>MAVNELLHLAPNVWPRNTTRDEVGVVCIAGIPLTQLAQEYGTPLFVIDEDDFRSRCRETAAAFGSGANVHYAAKAFLCSEVARWISEEGLCLDVCTGGELAVALHASFPPERITLHGNNKSVSELTAAVKAGVGHIVVDSMTEIERLDAIAGEAGIVQDVLVRLTVGVEAHTHEFISTAHEDQKFGLSVASGAAMAAVRRVFATDHLRLVGLHSHIGSQIFDVDGFELAAHRVIGLLRDVVGEFGPEKTAQIATVDLGGGLGISYLPSDDPPPIAELAAKLGTIVSDESTAVGLPTPKLVVEPGRAIAGPGTITLYEVGTVKD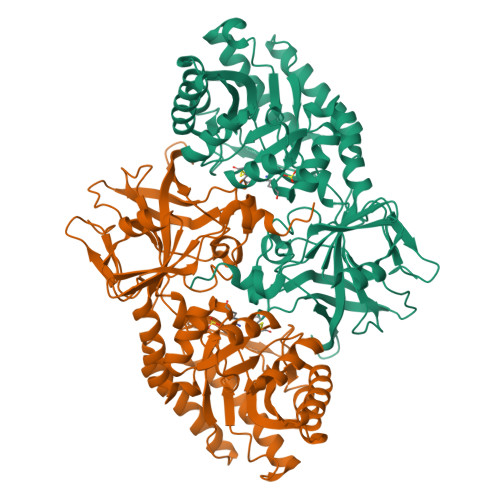VDVSATAHRRYVSVDGGMSDNIRTALYGAQYDVRLVSRVSDAPPVPARLVGKHCESGDIIVRDTWVPDDIRPGDLVAVAATGAYCYSLSSRYNMVGRPAVVAVHAGNARLVLRRETVDDLLSLEVRGVPRGKLAAALEHHHHHH[4x]N-methyl-3-(4-oxo-4,5-dihydrofuro[3,2-c]pyridin-2-yl)benzenesulfonamide 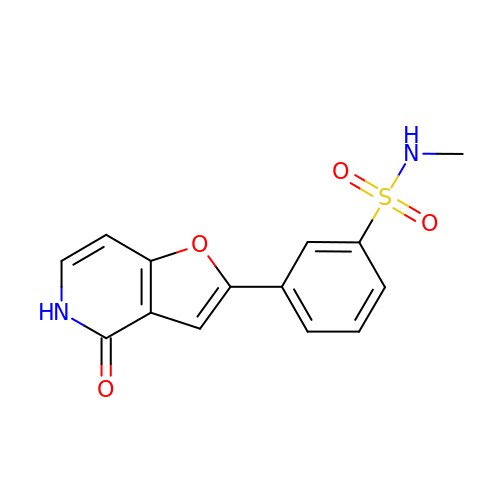| C14 H12 N2 O4 S | QWCULBJLWKNECO-UHFFFAOYSA-N>MGSEVEILKALLELKKSTAELKRATASLRAITEELKKNPSEDALVEHNRAIVEHNAIIVENNRIIAAVLMLIVVAVGMTQEIKKALEELVASTAELKRATASLRAITEELKKNPSEDALVEHNRAIVEHNAIIVENNRIIAAVLELIVRALNLTDAEVIKALIELRLSTLELVAATASLREITEELKKNPSEDALVEHNRAIVEHNAIIVENNRIIAAVLELIVGGSGGSGGSGGSSLEHHHHHH[20x]

Here we describe the de novo design of pH-responsive protein filaments built from subunits containing six or nine buried histidine residues that assemble into micrometre-scale, well-ordered fibres at neutral pH. We then applied the filament design method described in Shen et al. to dock these connected monomers into a wide variety of helical filament arrangements and design the amino acid residues at the newly formed interfaces to drive assembly.

All 18 designs were well expressed and soluble. Two designs (DpHF7 and DpHF18) were found to form filaments, as seen in negative stain electron microscopy (EM) images. We used cryogenic EM (cryo-EM) to determine the structures of DpHF7 and DpHF18 at high resolution. The resulting overall architecture can be viewed as a right-handed helix composed of two identical, parallel strands with contacting subunits. In contrast with the near-perfect agreement of the DpHF19 design model and the cryo-EM structure, the structure of DpHF7 differs considerably from the corresponding design model. The pH transition is thus reversible, and the pH transition midpoint can be increased by increasing the number of buried histidines. DpHF7 also has a reversible pH response, with disassembly at pH 4 and reassembly at pH 8.>GAMGSMSKQFVRSAKNLVKGYSSTQVLVRNATSNDNHQVSKDSLIELAEKSYDSADFFEIMDMLDKRLNDKGKYWRHIAKALTVIDYLIRFGSENCVLWCRENLYIIKTLKEFRHEDDEGIDQGQIVRVKAKELTALLSDDERLNEERNMNIKGRNRKGRRR[8x];>[8x]GAMGSMSRIDSDLQKALKKACSVEETAPKRKHVRACIVYTWDHQSSKAVFTTLKTLPLANDEVQLFKMLIVLHKIIQEGHPSALAEAIRDRDWIRSLGRVHSGGSSYSKLIREYVRYLVLKLDFHAHHRGFNNGTFEYEEYVSLVSVSDPDEGYETILDLMSLQDSLDEFSQIIFASIQSERRNTECKISALIPLIAESYGIYKFITSMLRAMHRQLNDAEGDAALQPLKERYELQHARLFEFYADCSSVKYLTTLVTIPKLPVDAPDVFLINDVDESKEIKFKKREPSVT

Throughout this process in yeast, endocytic coat adaptors, Sla2 and Ent1, must remain attached to the plasma membrane to transmit force from the actin cytoskeleton required for successful membrane invagination. Adaptors Ent1 and Sla2 co-assemble at the plasma membrane in a phosphatidylinositol 4,5-bisphosphate (PIP2)-dependent manner through their epsin N-terminal homology (ENTH) and AP180 N-terminal homology (ANTH) domains, respectively. Here, we present a cryo-EM structure of a 16-mer complex of the ANTH and ENTH membrane-binding domains from Sla2 and Ent1 bound to PIP2 that constitutes the anchor to the plasma membrane.

Focusing on the most abundant complex (16-mer), the structure reveals an assembly of 8 ANTH and 8 ENTH units arranged into four tetramers, each tetramer consisting of two molecules of ANTH and two of ENTH (A2E2). The global resolution of the final EM map is 3.9 Å (gold-standard Fourier shell correlation threshold 0.143) with analysis of the local resolution showing higher resolution towards the core of the map, reaching 3.7 Å. The cryo-EM map shows that each A2E2 tetramer contains three distinct lipid-binding sites, harboring 5 lipids per A2E2 with a total of 20 PIP2 lipids resolved in the entire 16-mer complex. PIP2 was found in three different binding sites, one in the ENTH domain, previously known from the crystal structure, one in the interface between the two ENTH domains of one tetramer, and one in the interface between the ANTH and ENTH domains, acting as a ‘glue’ for the oligomerization of both domains. Within each AENTH tetramer, the interactions between the ANTH and ENTH domains are established through two main hetero-dimerization interfaces and one homo-dimerization ANTH-ANTH interface. Our structure shows that ENTH T104 and ANTH R29 are located in one of the observed interfaces, defined as “ANTH-ENTH interface 1”. A second interface in the AENTH tetramer involves residues K10, K13, and K14 of ANTH. Altogether, these results indicate that lysines of the ANTH-ENTH interface 2 are essential for the assembly of the tetrameric lipid-binding AENTH unit and for the AENTH function in vivo. Since samples were prepared above the critical micelle concentration (CMC) of di-C8-PI(4,5)P238,39, the position of the polar groups indicates that the core of the map is composed of a PIP2 micelle around which the ANTH and ENTH domains assemble. Our tetrameric structure suggests a mechanism of lipid locking as the anchor unit to the membrane that would enable force transmission coming from actin polymerization for invagination to take place.>MAANLPLVVALDTEVLKAIDVAKRLKGAVAGFKVGWDLIFEGGISIVGEIARYGNVIVDLKIADVPHVASRVVEKLVNRGACCVIVHGFLHPSLPRGQHVYVLV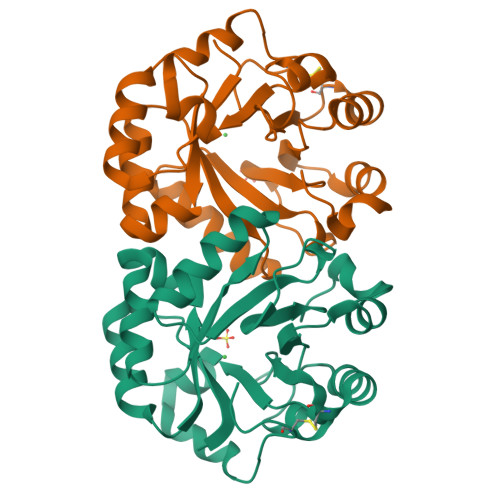KMTAPTIYDEMWEKLLNSVQDVRGFVLPGNQPEVVAQARKRIGCSYRIISPGIGPQGGRPGAAIEAGADFEIVGRYVLEDPARISQWAQYRPTCFETP[2x]>[4x]MGFK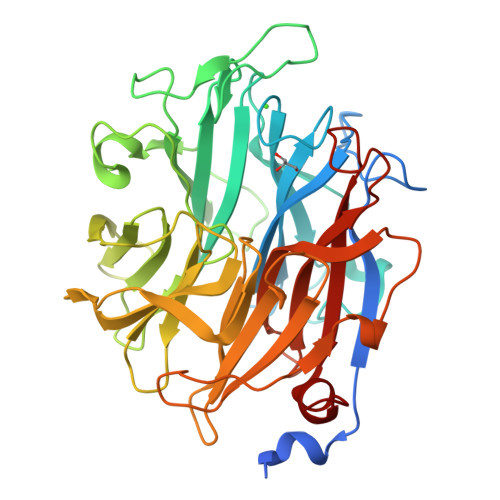QWLLSLAVVAFSATATQARVDDPAGKAAQYHKEYALFRSANMPSPDKLATGVGFHSFRIPAVVRTNTGRILAFAEGRRHNNRDYGDINLVYKRTKSPTNNGENPTDWESLREVVGTGPHTWGNPTPVVDGNTIYLFLSMNDGAYSQNGGNTLPDGTKTKKIDSTWVGRRHLYLTTSTDDGDTWTKPVDMTKTLTPDGQAWDAVGPGNGIKLSTGELVIPAQGRNIIGRGPSGNRTWSMQILKGAGSEGTICQTPDGKLMRNDRPGPMGHRSVARGTLAGLGPFATDNGLPDPACQGSILSYNSDEPARTIFMNSASTDRRTAMRVRISYDKDAAKFNFGRELKDAPLGNVGNEGGYSSMTKTSDYKIGALVESDWYEDKGGEKSHRCIIWRRFNLSWIINGPNN>MAHHHHHHMTSPALAPPQNTAEFWIKRLQLVPHPEGGYYSEVVRSAHKVDNEEGNRRHAYTTIYFLCTPESPSHLHRLCSDETWMYHAGDPLQLHVILKDPQDEDRIAAQPPAAPQAETDTADARPKYQVYRRVLVGARVERGELLQYTVPGGAIFGSSVAADGADGQAGYSLVSCIVSPGFDYRDFEIFTQAQLMELYPQHEAVIKQMAYETLPNHARLQ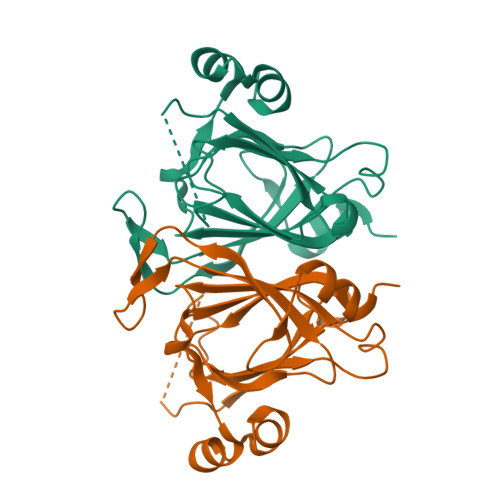TTEI[8x]>GHMNPIVELFIKDFTKEVMEENAAIFAGAGLSMSVGYVSWAKLLEPIAQEIGLDVNKENDLVSLAQYYCNENQGNRGRINQIILDEFSRKVDLTENHKILARLPIHTYWTTNYDRLIEKALEEENKIADVKYTVKQLATTKVKRDAVVYKMHGDVEHPSEAVLIKDDYEKYSIKMDPYIKALSGDLVSKTFLFVGFSFTDPNLDYILSRVRSAYERDQRRHYCLIKKEERRPDELEADFEYRVRKQELFISDLSRFNIKTIVLNNYNEITEILQRIENNIKTKTVFLSGSAVEYNHWETEHAEQFIHQLSKELIRKDFNIVSGFGLGVGSFVINGVLEELYMNQGTIDDDRLILRPFPQGKKGEEQWDKYRRDMITRTGVSIFLYGNKIDKGQVVKAKGVQSEFNISFEQNNYVVPVGATGYIAKDLWNKVNEEFETYYPGADARMKKLFGELNNEALSIEELINTIIEFVEILSN[4x]

The Thoeris system is composed of two genes, thsA and thsB. In the present study, we report structural and functional analyses of the ThsA and ThsB proteins from the B. cereus Thoeris defense system. Crystal structures of ThsA and ThsB were determined to resolutions of 2.5 and 1.8 Å, respectively. Combined with previous findings, these results advance our understanding of the molecular mechanism underlying the Thoeris defense system and suggest that NAD+ degradation is a previously unknown strategy for bacterial antiphage resistance.

To further investigate the role of ThsA in Thoeris-mediated phage defense, we determined the crystal structure of B. cereus ThsA. The asymmetric unit contains four ThsA protomers (chains A–D), the structures of which are essentially identical. The protomers form two dimeric assemblies (AB and CD), which are very similar to each other. Consistent with this prediction, SEC with multi-angle light scattering (MALS) analysis confirmed that the tetrameric state of ThsA is predominant in a solution containing a trace amount of octamer. The protomer structure of ThsA revealed a two-domain architecture that consists of an N-terminal sirtuin-like domain (residues 1–283) and a C-terminal SLOG-like domain (residues 284–476). The N-terminal domain contains the Rossmann-like fold, in which an extended seven-stranded parallel β-sheet (β3–β4–β2–β1–β5–β6–β7) is sandwiched between two helical layers (α1, α5, α6, and α11 on one side and α7–α10 on the other), comprising a three-layered globular structure. The acetyl substrate-binding pocket of sirtuins is not available in the N-terminal domain of ThsA due to the blocking by its α7 helix, excluding the possibility that ThsA serves as an NAD+-dependent deacetylase like sirtuins. A structural analysis indicated that this domain could be classified into the Sir2/TIR-associating SLOG (STALD) family within the SLOG superfamily. In our crystal structure of ThsA, this residue is found within the putative NAD+ binding site in its N-terminal domain. Using liquid chromatography–mass spectrometry (LC-MS), we identified nicotinamide (Nam) and adenosine-5ʹ-diphosphoribose (ADPR) as products of NAD+ degradation by ThsA, implying that ThsA cleaves NAD+ into Nam and ADPR by hydrolyzing the Nam–ribosyl bond of NAD+.> DRVTTQTAGNTAINTQSSLGVLCAYVEDPTKSDPPSSSTDQPTTTFTAIDRWYTGRLNSWTKAVKTFSFQAVPLPGAFLSRQGGLNGGAFTATLHRHFLMKCGWQVQVQCNLTQFHQGALLVAMVPETTLDVKPDGKAKSLQELNEEQWVEMSDDYRTGKNMPFQSLGTYYRPPNWTWGPNFINPYQVTVFPHQILNARTSTSVDINVPYIGETPTQSSETQNSWTLLVMVLVPLDYKEGATTDPEITFSVRPTSPYFNGLRNRY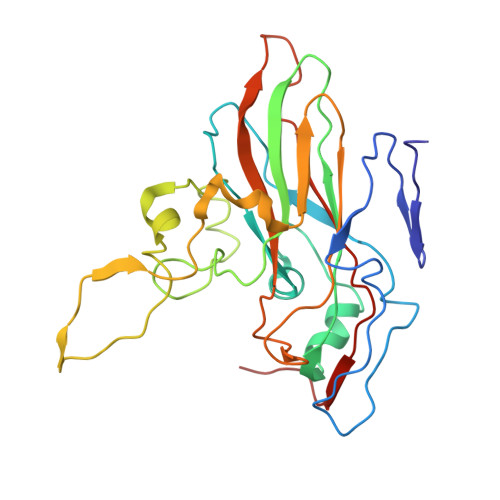TT> NEGCAPLTGKESGMDIGRSSTERCLPGANPLQDQQWYLLNSGQDGFSARGGIAGNDLNLWWAHRTGVLGQGVNVAVVDDGLAIAHPDLADNVRPGSKNVVTGSDDPTPTDPDTAHGTSVSGIIAAVDNAIGTKGIAPRAQLQGFNLLDDNSQQLQKDWLYALGDSNASRDNRVFNQSYGMSVVDPRSANSLDQSQLDRLFEQQTLKAQGAAYIKAAGNGFNKIAAGGYVLNR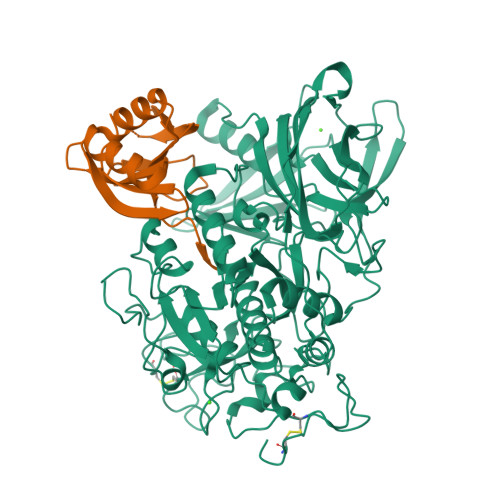TGNGPKLPFENSNLDPSNSNFWNLVVSALNADGVRSSYSSVGSNIFLSATGGEYGTDTPAMVTTDLPGCDMGYNRTDDPSTNRLHGNSQLDASCDYNGVMNGTASATPSTSGAMALLMSAYPDLSVRDLRDLLARSATRVDAKHQPVMVSYTSSTGKVRDVKGLEGWERNAAGMWFSPTYGFGLIDVNKALELAANHQPLPPLVQLPWQKINVTGSAAAIADVGNSPTSSTTRIATPLTVEAVQVMVSLDHQRLPDLLIELVSPAGTRSILLSPFNSLVGQSLDQQQLGFVRTKGLRDMRMLSNKFYGESAQGTWRLEVTDVANGTRQVSLLNRETRERTTLTERNNRQPGKLISWSLRVLGHDANRS;> QEHHHHHHSSGLVPRGSGQESVTMDGKQYSTIEVNGQTYLIPDNGSKKRVARSLDSKVPQQTLRRGDVLMQGAASPELTVSGTLLVEADDASAKALATRHGLNFKQSSGGIALLEAKPGTDLNAIATKLKSEGVNVQIELSGAEQQPK>[2x]VKIVTVKTKAYPDQKPGTSGLRKRVKVFQSSTNYAENFIQSIISTVEPAQRQEATLVVGGDGRFYMKEAIQLIVRIAAANGIGRLVIGQNGILSTPAVSCIIRKIKAIGGIILTASHNPGGPNGDFGIKFNISNGGPAPEAITDKIFQISKTIEEYAICPDLKVDLGVLGKQQFDLENKFKPFTVEIVDSVEAYATMLRNIFDFNALKELLSGPNRLKIRIDAMHGVVGPYVKKILCEELGAPANSAVNCVPLEDFGGHHPDPNLTYAADLVETMKSGEHDFGAAFDGDGDRNMILGKHGFFVNPSDSVAVIAANIFSIPYFQQTGVRGFARSMPTSGALDRVANATKIALYETPTGWKFFGNLMDASKLSLCGEESFGTGSDHIREKDGLWAVLAWLSILATRKQSVEDILKDHWHKFGRNFFTRYDYEEVEAEGATKMMKDLEALMFDRSFVGKQFSANDKVYTVEKADNFEYHDPVDGSVSKNQ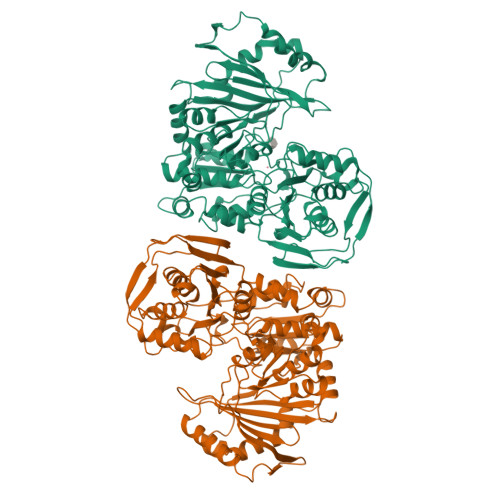GLRLIFADGSRIIFRLSGTGSAGATIRLYIDSYEKDNAKINQDPQVMLAPLISIALKVSQLQERTGRTAPTVIT>AAVIEKRATCSNGKTVGDASCCAWFDVLDDIQQNLFHGGQCGAEAHESIRLVFHDSIAISPAMEAQGKFGGGGADGSIMIFDDIETAFHPNIGLDEIVKLQKPFVQKHGVTPGDFIAFAGAVALSNCPGAPQMNFFTGRAPATQ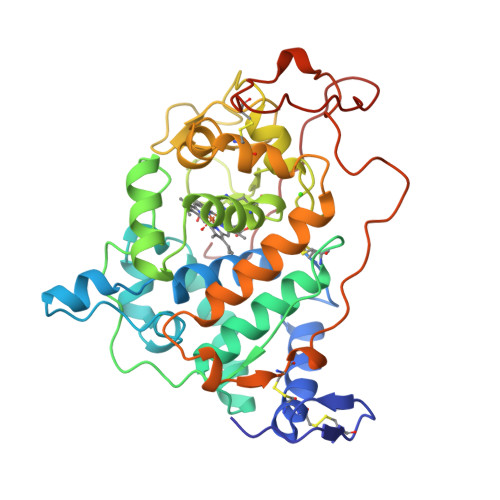PAPDGLVPEPFHTVDQIINRVNDAGEFDELELVWMLSAHSVAAVNDVDPTVQGLPFDSTPGIFDSQFFVETQLRGTAFPGSGGNQGEVESPLPGEIRIQSDHTIARDSRTACEWQSFVNNQSKLVDDFQFIFLALTQLGQDPNAMTDCSDVIPQSKPIPGNLPFSFFPAGKTIKDVEQACAETPFPTLTTLPGPETSVQRIPPPPGA[2x]>GPVVLSTPAQLIAPVVVAKGTLSITTTEIYFEVDEDDSAFKKIDTKVLAYTEGLHGKWMFSEIRAVFSRRYLLQNTALEVFMANRTSVMFNFPDQATVKKVVYSLPRVGVGTSYGLPQARRISLATPRQLYKSSNMTQRWQRREISNFEYLMFLNTIAGRTYNDLNQYPVFPWVLTNYESEELDLTLPGNFRDLSKPIGALNPKRAVFYAERYETWEDDQSPPYHYNTHYSTATSTLSWLVRIEPFTTFFLNANDGKFDHPDRTFSSVARSWRTSQRDT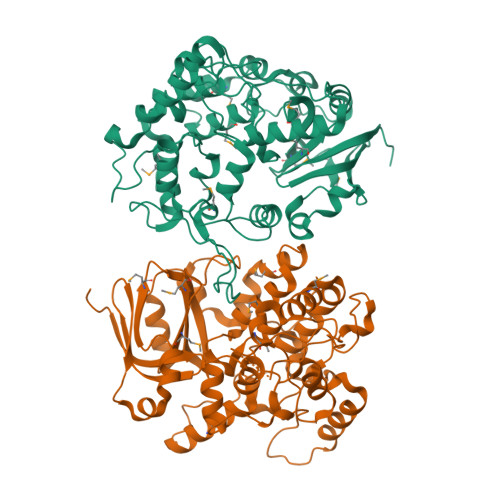SDVKELIPEFYYLPEMFVNSNGYNLGVREDEVVVNDVDLPPWAKKPEDFVRINRMALESEFVSCQLHQWIDLIFGYKQRGPEAVRALNVFHYLTYEGSVNLDSITDPVLREAMEAQIQNFGQTPSQLLIEPHPPR[2x]>[4x]MISNSSAESISAPPNDSTIPHLAIDPFSLDFFDDPYPDQQTLRDAGPVVYLDKWNVYGVARYAEVHAVL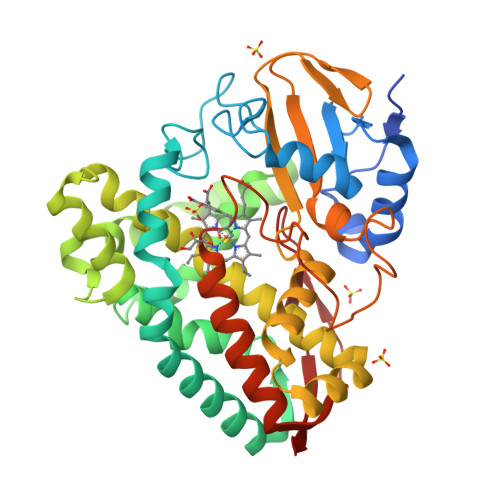NDPTTFCSSRGVGLSDFKKEKPWRPPSLILEADPPAHTRPRAVLSKVLSPATMKTIRDGFAAAADAKVDELLQRGCIDAIADLAEAYPLSVFPDAMGLKQEGREHLLPYAGLVFNAFGPPNELRQTAIERSAPHQAYVNEQCQRPNLAPGGFGACIHAFTDTGEITPDEAPLLVRSLLSAGLDTTVNGIGAAVYCLARFPGELQRLRSDPTLARNAFEEAVRFESPVQTFFRTTTREVELGGAVIGEGEKVLMFLGSANRDPRRWSDPDLYDITRKTSGHVGFGSGVHMCVGQLVARLEGEVMLSALARKVAAIDIDGPVKRRFNNTLRGLESLPVKLTPA2-(2-carboxyethyl)-1,1,1-trimethyldiazanium 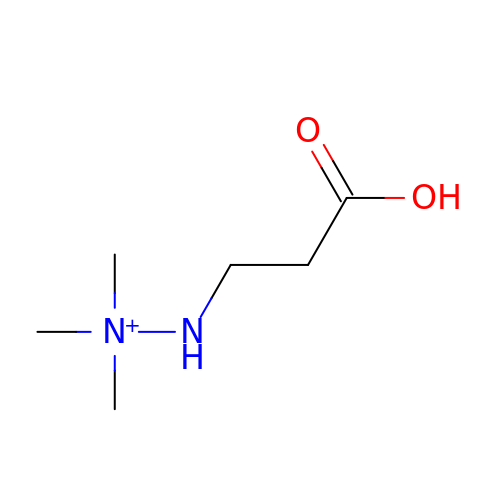| C6 H15 N2 O2 | PVBQYTCFVWZSJK-UHFFFAOYSA-O> MQDTIFLKGMRFYGYHGALSAENEIGQ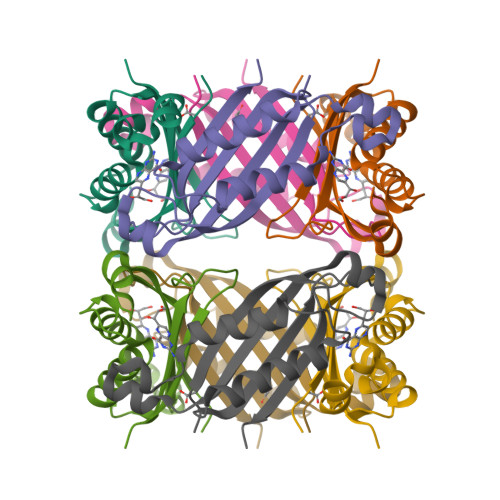IFKVDVTLKVDLSEAGRTDNVIDTVHYGEVFEEVKSIMEGKAVNLLEHLAERIANRINSQYNRVMETKVRITKENPPIPGHYDGVGIEIVRENK>[2x]EPTCNTPSNRACWSDGFDINTDYEVSTPDTGVTQSYVFNLTEVDNWMGPDGVVKEKVMLINGNIMGPNIVANWGDTVEVTVINNLVTNGTSIHWHGIHQKDTNLHDGANGVTECPIPPKGGQRTYRWRA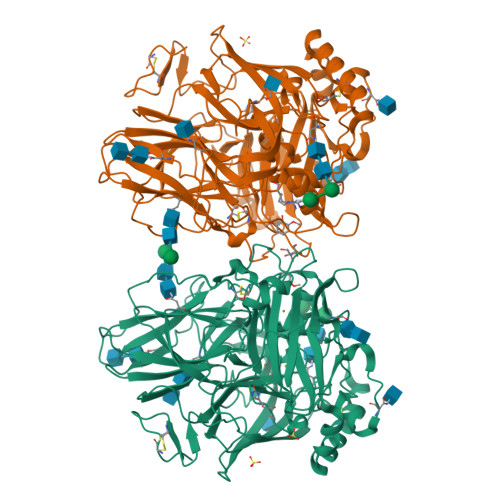RQYGTSWYHSHFSAQYGNGVVGTIQINGPASLPYDIDLGVFPITDYYYRAADDLVHFTQNNAPPFSDNVLINGTAVNPNTGEGQYANVTLTPGKRHRLRILNTSTENHFQVSLVNHTMTVIAADMVPVNAMTVDSLFLAVGQRYDVVIDASRAPDNYWFNVTFGGQAACGGSLNPHPAAIFHYAGAPGGLPTDEGTPPVDHQCLDTLDVRPVVPRSVPVNSFVKRPDNTLPVALDLTGTPLFVWKVNGSDINVDWGKPIIDYILTGNTSYPVSDNIVQVDAVDQWTYWLIENDPEGPFSLPHPMHLHGHDFLVLGRSPDVPAASQQRFVFDPAVDLARLNGDNPPRRDTTMLPAGGWLLLAFRTDNPGAWLFHCHIAWHVSGGLSVDFLERPADLRQRISQEDEDDFNRVCDEWRAYWPTNPYPKIDSGL(8S)-5-(2-aminopyrimidin-4-yl)-N-[2-(dimethylamino)ethyl]-4,5,6,7-tetrahydropyrazolo[1,5-a]pyrazine-2-carboxamide 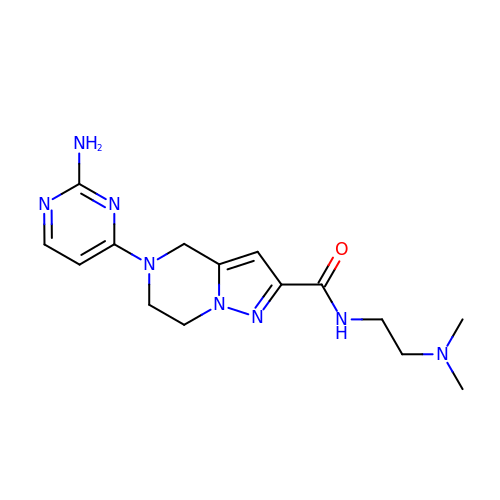| C15 H22 N8 O | SOQWCHRGAQNWSN-UHFFFAOYSA-N> LLNFDELPEPPATFCDPEEVEG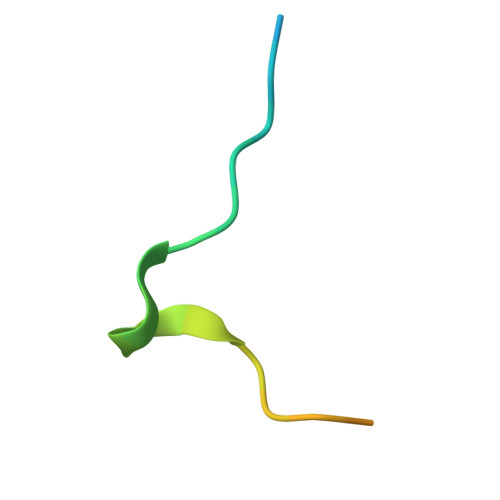SGENLQ Type IIB receptor protein tyrosine phosphatases are cell surface transmembrane proteins that engage in cell adhesion via their extracellular domains (ECDs) and cell signaling via their cytoplasmic phosphatase domains. The four human R2B RPTPs (PTPRK, PTPRM, PTPRT, and PTPRU) are type 1 transmembrane proteins and share a common extracellular domain (ECD) architecture of one MAM (meprin/A5/μ), one immunoglobulin (Ig)-like, and four fibronectin (FN) type-III domains, with the most membrane proximal FN domain undergoing furin cleavage in the secretory pathway. Previous studies have shown that PTPRK, PTPRM, and PTPRT form homodimers, but not heterodimers, in cell aggregation assays. The homophilic (trans) interactions of R2B RPTPs determine their subcellular localization and have been proposed to function as spacer clamps between cell membranes.

Crystals grew in two space groups, P212121 and P3221, possessing two and four molecules per asymmetric unit, respectively. All six chains are essentially identical in structure (pairwise RMSDs over 220 Cα atoms range from 0.44 to 0.92 Å). The main difference between the protein structures is that one chain in the P212121 crystal has a disordered loop (residues 628–641) that in all other chains was ordered via intermolecular interactions. This loop is anchored at one end via a disulfide bond within the FN4 domain (C642 to C716), and the sequence encompasses the furin-cleavage site of PTPRM, illustrating that this site is surface accessible within a conformationally dynamic loop, but that cleavage would not significantly destabilize the fold of the FN4 domain. In both crystal forms, one chain is missing the glycan on N598, indicating that PTPRM-FN4 not only adopts conformational differences in the furin-cleavage loop but also can undergo heterogeneous glycosylation. Although the previous structure of the PTPRM ECD had no interpretable electron density for the FN4 domain, it was present in the construct. Superposition of the FN3 domains from our structure with this previous PTPRM structure demonstrates that the FN4 domain can be accommodated without significant steric clashes with surrounding chains, and FN4 colocalizes with weak and disconnected electron density that is unmodeled in the deposited structure.

>ETGDEDLPGAVPTESIQGSTFEEKIFLQWREPTQTYGVITLYEITYKAVSSFDPEIDLSNQSGRVSKLGNETHFLFFGLYPGTTYSFTIRASTAKGFGPPATNQFTTKISAPSMPAYELETPLNQTDNTVTVMLKPAHSRGAPVSVYQIVVEEERPRRTKKTTEILKCYPVPIHFQNASLLNSQYYFAAEFPADSLQAAQPFTIGDNKTYNGYWNTPLLPYKSYRIYFQAASRANGETKIDCVQVATKGGTKHHHHHH[4x]> MLDNPFIGAIGYVNPDWATNVISQANQTADPTLAAQMRKVATYSTAVWLDRIAAITAGRGLRGHLDEALRQMQQAGQPVVITLVIYDLPNRDCSAAASNGELLVAQNGLARYKAEFIDPIVAILSDPRYAGLRIVTIIEPDSLPNLVTNLSIPACAEAQNAYIEGIRYAVNRLRTIPNVYIYLDIAHSGWLGWDNNFNGAVNLYTQVVQGMDQGFNSIDGFITNVANYTPLEEPYLPDPNLTIAGQPVRSASFYEWNPYFDELDYALALRNAFIGRGFPSTIGMLIDTSRNGWGGCSYGRCRPTGPSSDTSSVNAYVDGSRVDRRYHRGNWCNQAGGIGERPQAAPRSGIDAYVWVKPPGESDGVSQPGIVDPDDPNKKFDPMCDPNGQSRYNSAYPTGALPNAPHAGRWFPQQF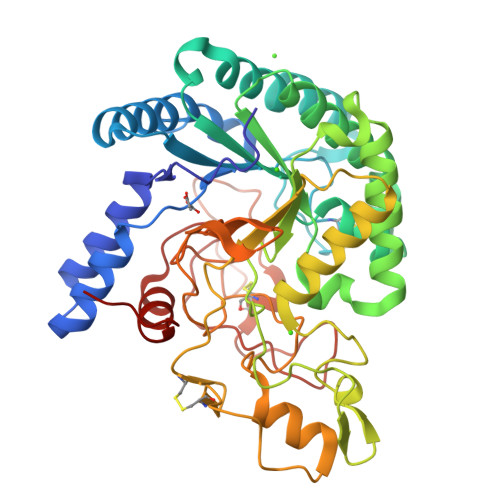EILVRNAYPPIQP>[4x]MASDVTVNVSAEKQVIRGFGGMNHPAWAGDLTAAQRETAFGNGQNQLGFSILRIHVDENRNNWYKEVETAKSAVKHGAIVFASPWNPPSDMVETFNRNGDTSAKRLKYNKYAAYAQHLNDFVTFMKNNGVNLYAISVQNEPDYAHEWTWWTPQEILRFMRENAGSINARVIAPESFQYLKNL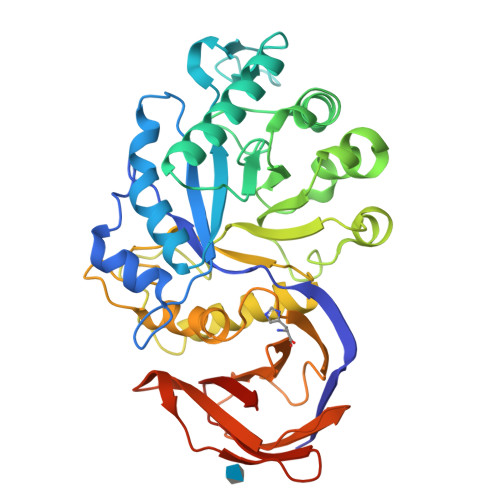SDPILNDPQALANMDILGTHLYGTQVSQFPYPLFKQKGAGKDLWMTEVYYPNSDTNSADRWPEALDVSQHIHNAMVEGDFQAYVWWYIRRSYGPMKEDGTISKRGYNMAHFSKFVRPGYVRIDATKNPNANVYVSAYKGDNKVVIVAINKSNTGVNQNFVLQNGSASNVSRWITSSSSNLQPGTNLTVSGNHFWAHLPAQSVTTFVVNRLEHHHHHHHH> MIVLFVDFDYFYAQVEEVLNPSLKGKP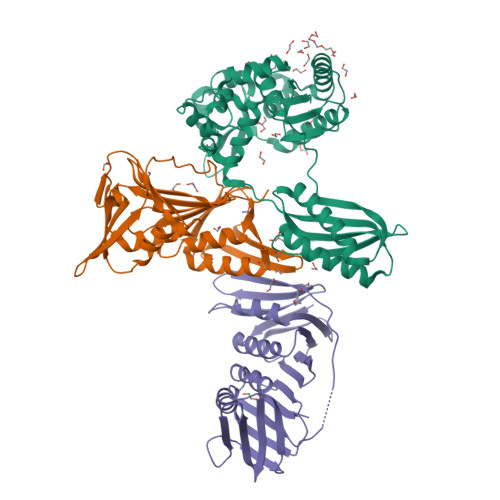VVVCVFSGRFEDSGAVATANYEARKFGVKAGIPIVEAKKILPNAVYLPMRKEVYQQVSSRIMNLLREYSEKIEIASIDEAYLDISDKVRDYREAYNLGLEIKNKILEKEKITVTVGISKNKVFAKIAADMAKPNGIKVIDDEEVKRLIRELDIADVPGIGNITAEKLKKLGINKLVDTLSIEFDKLKGMIGEAKAKYLISLARDEYNEPIRTRVRKSIGRIVTMKRNSRNLEEIKPYLFRAIEESYYKLDKRIPKAIHVVAVTEDLDIVSRGRTFPHGISKETAYSESVKLLQKILEEDERKIRRIGVRFSKFIEAIGLDKFFDT;> MVKIVYPNAKDFFSFINSITNVTDSIILNFTEDGIFSRHLTEDKVLMAIMRIPKDVLSEYSIDSPTSVKLDVSSVKKILSKASSKKATIELTETDSGLKIIIRDEKSGAKSTIYIKAEKGQVEQLTEPKVNLAVNFTTDESVLNVIAADVTLVGEEMRISTEEDKIKIEAGEEGKRYVAFLMKDKPLKELSIDTSASSSYSAEMFKDAVKGLRGFSAPTMVSFGENLPMKIDVEAVSGGHMIFWIAPRL;> MMKAKVIDAVSFSYILRTVGDFLSEANFIVTKEGIRVSGIDPSRVVFLDIFLPSSYFEGFEVSQEKEIIGFKLEDVNDILKRVLKDDTLILSSNESKLTLTFDGEFTRSFELPLIQVESTQPPSVNLEFPFKAQLLTITFADIIDELSDLGEVLNIHSKENKLYFEVIGDLSTAKVELSTDNGTLLEASGADVSSSYGMEYVANTTKMRRASDSMELYFGSQIPLKLRFKLPQEGYGDFYIAPRA>GGCCAATTGG[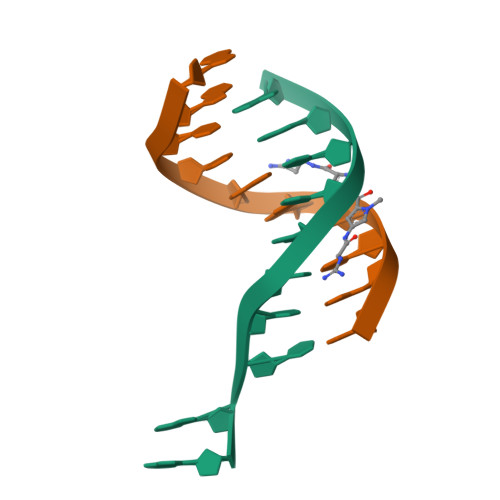2x]> AGIAAKLAKDREAAEGLGSHERAIKYLNQDYEALRNECLEAGTLFQDPSFPAIPSALGFKELGPYSSKTRGMRWKRPTEICADPQFIIGGATRTDICQGALGDCWLLAAIASLTLNEEILARVVPLNQSFQENYAGIFHFQFWQYGEWVEVVVDDRLPTKDGELLFVHSAEGSEFWSALLEKAYAKINGCYEALSGGATTEGFEDFTGGIAEWYELKKPPPNLFKIIQKALQKGSLLGCSIDITSAADSEAITFQKLVKGHAYSVTGAEEVESNGSLQKLIRIRNPWGEVEWTGRWNDNCPSWNTIDPEERERLTRRHEDGEFWMSFSDFLRHYSRLEICNLTPDTLTSDTYKKWKLTKMDGNWRRGSTAGGCRNYPNTFWMNPQYLIKLEEEDEDEEDGESGCTFLVGLIQKHRRRQRKMGEDMHTIGFGIYEVPEELSGQTNIHLSKNFFLTNRARERSDTFINLREVLNRFKLPPGEYILVPSTFEPNKDGDFCIRVFSEKKADYQAVDDEIEANLEEFDISEDDIDDGVRRLFAQLAGEDAEISAFELQTILRRVLAKRQDIKSDGFSIETCKIMVDMLDSDGSGKLGLKEFYILWTKIQKYQKIYREIDVDRSGTMNSYEM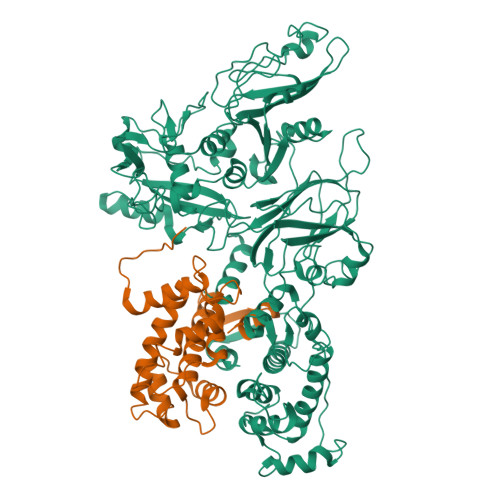RKALEEAGFKMPCQLHQVIVARFADDQLIIDFDNFVRCLVRLETLFKIFKQLDPENTGTIELDLISWLCFSVL;> THYSNIEANESEEVRQFRRLFAQLAGDDMEVSATELMNILNKVVTRHPDLKTDGFGIDTCRSMVAVMDSDTTGKLGFEEFKYLWNNIKRWQAIYKQFDTDRSGTICSSELPGAFEAAGFHLNEHLYNMIIRRYSDESGNMDFDNFISCLVRLDAMFRAFKSLDKDGTGQIQVNIQEWLQLTMYS>[8x]MNHKVHHHHHHIEGRHMITKEERAQINADPELGAGNVLHRLRAYGRPTDRPVLWTDGTWRAPDGSHPEVITLGELYEYVETYAGFYHGKGIRPRDVVGVLTASSTEFAINFMAINSLGAIPSFANAKLRPEIAREYIRRQGASGAVTDTERHEVLAGGELGFVVTAEDIRPEHRAQLPQGWPYRHDPTDPIIISHSSGTTGMPKAVPHTHQTLLYAQLHRLKLSVGGSMGRLLVALPGNHNAAMSVMMFGLLLDSPVYLQSSQRGSDVLDAIEKFKPTTVFGFSGTYGQIATSDLSTRDMSSIEAYYNTGDAAHEAHIRVLVAQGSHEEIGPDFKPVRVPGSVFTDGLGSSETGYSIFHNGHKPGSASFGRCIGKPMSFAQAAVLSEDGRPLPAGEVGRLGVRSPTLTPGYWNDSLTWHKLRLGGYWLTGDLAMQDAEGNFYHLDRAPDAIRTEAGI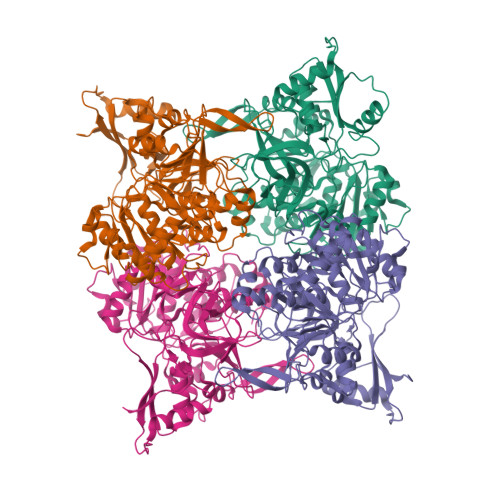VFSTRTEELLLASLPELADCTVTAIAEEGVRADWDGDGVAEAYVLLQFTDGAREPGDLTGWVNEVLAGQGFPPVTRALRMDSTDVSTGVTGKVLKRVMRERARELVARADQG> GPLGSMADEATRRVVSEIPVLKTNAGPRDRELWVQRLKEEYQSLIRYVENNKNADNDWFRLESNKEGT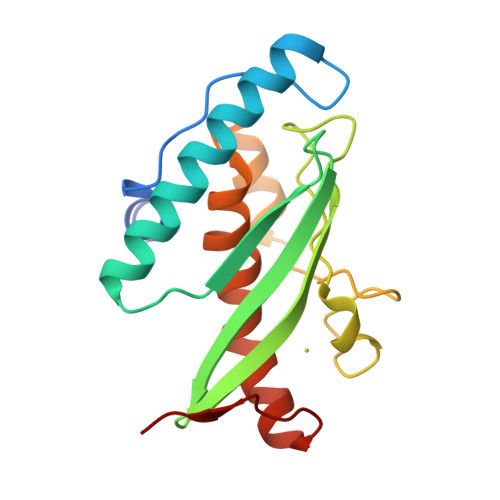RWFGKCWYIHDLLKYEFDIEFDIPITYPTTAPEIAVPELDGKTAKMYRGGKICLTDHFKPLWARNVPKFGLAHLMALGLGPWLAVEIPDLIQKGVIQHKEKCNQ>[3x]MQISSDYIPD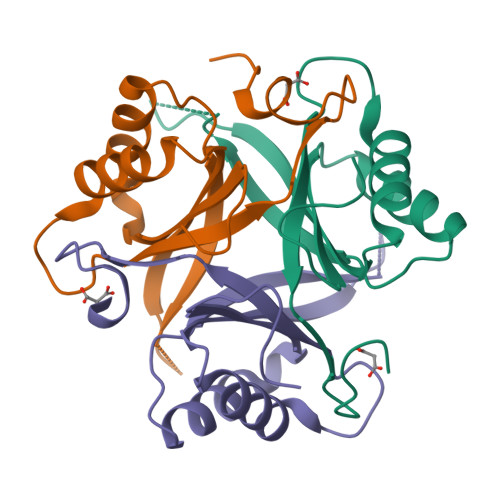SKFYKVEAIVRPWRIQQVSSALLKIGIRGVTVSDVRGFGAQGGSTERHGGSEFSEDKFVAKVKMEIVVKKDQVESVINTIIEGARTGEIGDGKIFVLPVSDVIRVRTGERGEKAEKMTGDMLSPS>HMSTQPKTL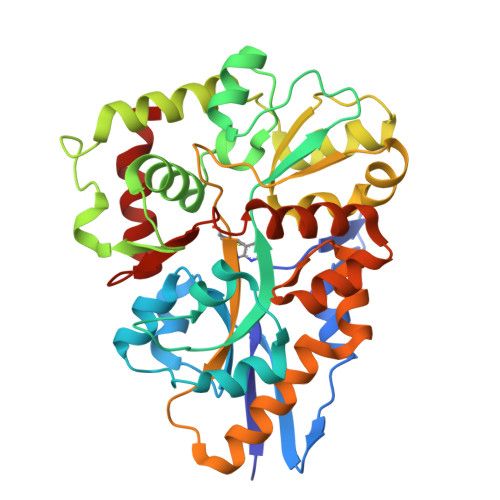TVGLFPYLPSWNENGNEVKLINLIKDVLPTQVSGYNIEYTEFDCYSDASLQSLPDVFSTDSIFLPYLVSLGGVKSLDESLVRGVTGDLHSFVSSSASVNGSVYGFPQYLCSNFLLSSPNATQQASSLLELAQKVGYEQIVYPDVASSSSFTVFGLYQQLLQSSSSAAVDIKASDLPQSGDQVNKDITQKYRTILDSTVVASQREYINSVKQGKPISNYYVGYSESMCEIKDIIRDQQYNVQLIGTSDKPYVYTDVLALNSNLCDEKQKVAVEVIKNLLTNTLVLDLLGLGLTLPANKNGIAHLAKSSNFYAQLSQQFDAKESEVRVLRCVDFANKEVKNCAGVLRPFL[6x]>[2x]MVTSPALRDVHVPHAYPEQQVDLGEITMNYAEAGDPDRPAVLLIPEQTGSWWSYEEAMGLLSEHFHVYAVDLRGQGRSSWTPKRYSLDNFGNDLVRFIALVVKRPVVVAGNSSGGVLAAWLSAYSMPGQLRGVLCEDPPFFASELVPAHGHSVRQGAGPVFELFRTYLGDQWSVGDWEGFCRAAGASASPMARSFVADGIPQHLQEYDPEWARVFYEGTVGLSCPHERMLGQVKTPVLLTHHMRGIDPETGNLLGALSDEQALRARRLMDSAGVTVDYESVPDASHMMHQSAPARYVEIFTRWAAALAPHHHHHH

Zearalenone (ZEN) is a mycoestrogenic polyketide produced by Fusarium graminearum and other phytopathogenic members of the genus Fusarium. ZenA cleaves zearalenone [ZEN, (S,E)-14,16-dihydroxy-3-methyl-3,4,5,6,9,10-hexahydro-1H-benzo[c][1]oxacyclotetradecine-1,7(8H)-dione] to hydrolyzed zearalenone [HZEN, (S,E)-2,4-dihydroxy-6-(10-hydroxy-6-oxoundec-1-en-1-yl)benzoic acid], which decarboxylates spontaneously to decarboxylated hydrolyzed zearalenone [DHZEN, (S,E)-1-(3,5-dihydroxyphenyl)-10-hydroxyundec-1-en-6-one]. Furthermore, we report site-directed mutagenesis as well as structural analysis of the dimeric ZenARe of R. erythropolis and the more thermostable, tetrameric ZenAScfl of Streptomyces coelicoflavus with and without bound ligands. The X-ray crystal structures not only revealed canonical features of α/β hydrolases with a cap domain including a Ser-His-Asp catalytic triad but also unusual features including an uncommon oxyanion hole motif and a peripheral, short antiparallel β-sheet involved in tetramer interactions.

The ZenAScfl tetramer is a dimer of dimers, and its subunits display canonical features of the α/β hydrolase fold. The core domain features a central β-sheet made of eight strands, which are parallel except for strand β2, which is inverted. This twisted β-sheet is sandwiched between two α-helices (A and F) on the front side and four α-helices (B, C, D, and E) on the back side. ZenAScfl features a cap domain inserted between sheet β6 and helix αD, composed of four α-helices. Notably, ZenAScfl features a β-sheet formed by two short, antiparallel strands linked by a tight turn between β-strand 7 and α-helix E, which protrudes from the α/β hydrolase core and touches the left side of the cap domain. We nicknamed this peculiar β-sheet, the “flake”. The catalytic triad of ZenAScfl is located in negatively charged cavities opposite the dimer interface and is composed of Ser-112, Asp-137, and His-286. The structure of ZenAScfl confirmed conserved His-286 in the loop between β-strand 8 and α-helix F as the catalytic histidine, at a distance of 2.9 Å between NE2 and OG of Ser-112. The crystal structure showed Asp-137 OD2 positioned at a distance of 2.7 Å from ND1 of the catalytic His-286. The backbone amides NH of Ser-113 and Gln-47 are in positions that suggest their functional role as hydrogen bond donors of the oxyanion hole of ZenAScfl.> MKSVLFLALAGSAAAFAPSTQSRSNTLLKADLSSLPGSTAPVGPFDPLNLADSGSEETLAWFRASELKHGRVAMLATTGYLVQG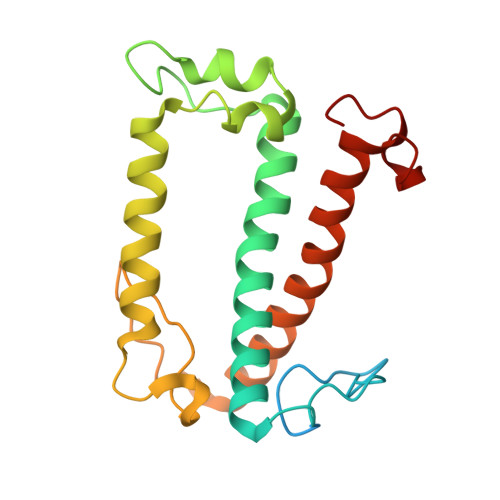AGIHFPGMLSSDVSFESLSAMKPLEAWDAVPDAGKAQILGTIFIAEMITESKPVHYTKGGPMPTMVFPAIDFSGVDAATLKRKQDSELNNGRLAMIAIMSFISAANIPGSVPALTNNPAF>DTGERRCDPIRISMCQNLGYNVTKMPNLVGHELQTDAELQLTTFTPLIQYGCSSQLQFFLCSVYVPMCTEKINIPIGPCGGMCLSVKRRCEPVLKEFGFAWPESLNCSKFPPQNDHNHMCMEGPGDEEVPLPHKTPIQPGEGTLE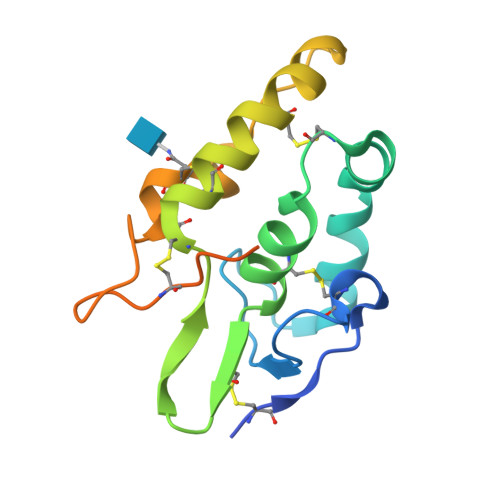VLFQ[4x]>[2x]SRPLSDQEKRKQISVRGLAGVENVTELKKNFNRHLHFTLVKDRNVATPRDYYFALAHTVRDHLVGRWIRTQQHYYEKDPKRIYYLSLEFYMGRTLQNTMVNLALENACDEATYQLGLDMEELEEIEEDAGLGNGGLGRLAACFLDSMATLGLAAYGYGIRYEFGIFNQKICGGWQMEEADDWLRYGNPWEKARPEFTLPVHFYGRVEHTSQG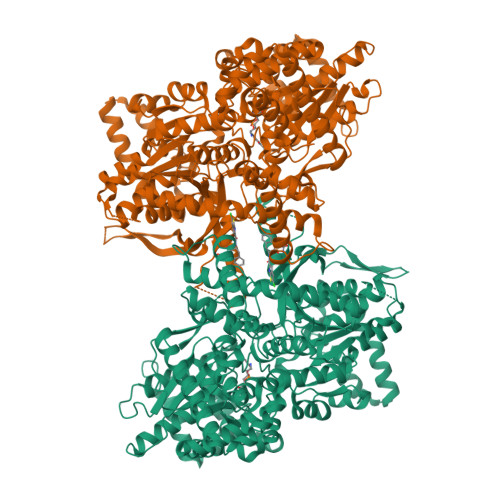AKWVDTQVVLAMPYDTPVPGYRNNVVNTMRLWSAKAPNDFNLKDFNVGGYIQAVLDRNLAENISRVLYPNDNFFEGKELRLKQEYFVVAATLQDIIRRFKSSKFGCRDPVRTNFDAFPDKVAIQLNDTHPSLAIPELMRVLVDLERLDWDKAWEVTVKTCAYTNHTVIPEALERWPVHLLETLLPRHLQIIYEINQRFLNRVAAAFPGDVDRLRRMSLVEEGAVKRINMAHLCIAGSHAVNGVARIHSEILKKTIFKDFYELEPHKFQNKTNGITPRRWLVLCNPGLAEIIAERIGEEYISDLDQLRKLLSYVDDEAFIRDVAKVKQENKLKFAAYLEREYKVHINPNSLFDVQVKRIHEYKRQLLNCLHVITLYNRIKKEPNKFVVPRTVMIGGKAAPGYHMAKMIIKLITAIGDVVNHDPVVGDRLRVIFLENYRVSLAEKVIPAADLSEQISTAGTEASGTGNMKFMLNGALTIGTMDGANVEMAEEAGEENFFIFGMRVEDVDRLDQRGYNAQEYYDRIPELRQIIEQLSSGFFSPKQPDLFKDIVNMLMHHDRFKVFADYEEYVKCQERVSALYKNPREWTRMVIRNIATSGKFSSDRTIAQYAREIWGVEPSRQRLPAPDEKIP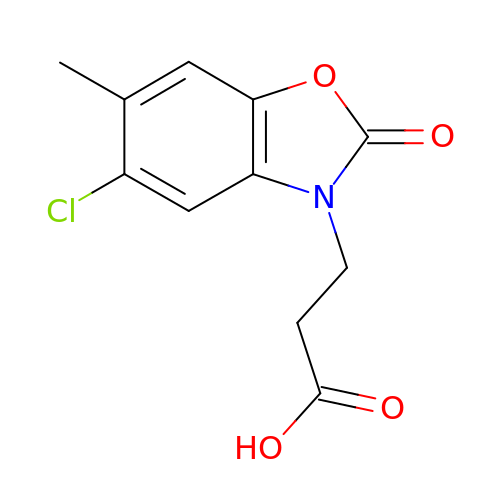3-(5-chloranyl-6-methyl-2-oxidanylidene-1,3-benzoxazol-3-yl)propanoic acid | C11 H10 Cl N O4 | QPMPFAMMRAXUAV-UHFFFAOYSA-N>MAAYTLPQLPYAYDALEPHIDARTMEIHHTKHHQTYVDNANKALEGTEFADLPVEQLIQQLDRVPADKKGALRNNAGGHANHSMFWQIMGQGQGQNGANQPSGELLDAINSAFGSFDAFKQKFEDAAKTRFGSGWAWLVVKDGKLDVVSTA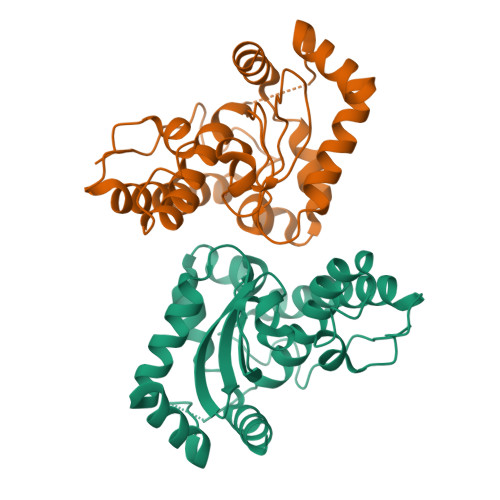NQDNPLMGEAIAGVSGTPILGVDVWEHAYYLNYQNRRPDYLAAFWNVVNWDEVSKRYAAAKLVPRGSAAALEHHHHHH[4x]> HMNKKILVVDDEESIVTLLQYNLERSGYDVITASDGEEALKKAETEKPDLI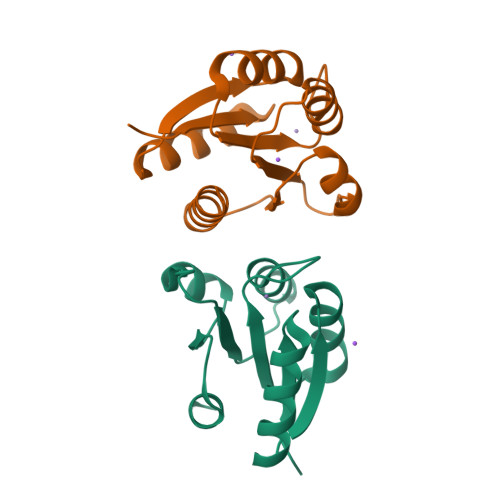VLDVMLPKLDGIEVCKQLRQQKLMFPILMLTAKDEEFDKVLGLELGADDYMTKPFSPREVNARVKAILRRSEIRAPSSEMKNDEM Glutaryl-CoA dehydrogenase (GCDH) is an acyl-CoA dehydro­genase (ACDH) which catalyzes an intermediate step in the metabolic breakdown of lysine and tryptophan. Unlike other flavoproteins within this family, GCDH (EC 1.3.99.7) performs α,β-dehydrogenation as well as decarboxylation of its sub­strate glutaryl-CoA to yield the product crotonyl-CoA. Transfer of electrons from the glutaryl-CoA precursor to the electron-transfer flavoprotein is mediated by the cofactor flavin adenine dinucleotide (FAD) in both prokaryotic and eukaryotic electron-transport chains. Like other ACDHs, GCDH from B. pseudomallei (BpGCDH) exists as a homotetramer with tetrahedral symmetry and possesses an overall fold similar to that of the human enzyme.

Additional structures of BpGCDH resulting from this effort were obtained by soaking apo BpGCDH crystals in drops containing our Fragments of Life (FOL) ligand collection prior to data collection. All fragments identified by screening which bind BpGCDH occupy the pockets that bind the glutaryl and flavin moieties of the substrate and cofactor, respectively. In three of the four ligand-bound complexes fragment molecules occupy the binding site for the terminal glutamate of the glutaryl-coenzyme A substrate. The crystallographic water coordinated to the Arg97 side chain in the apo structure of BpGCDH remains in place when FOL544 is bound, but is displaced by FOL239 and FOL6421. In all three of these cases the Tyr373 side chain is rotated approximately 90° from its position in both the apo BpGCDH structure and the human ternary complex. This new position appears to facilitate ligand binding by providing a parallel aromatic surface that aligns with the heteroaromatic rings of all three fragments. However, a conserved backbone deviation is observed between the structure of apo BpGCDH and those of all four fragment-bound complexes in this same region. In all four fragment-bound structures Thr376 and His377 are flipped out of the α-helix observed in the apo state, partially occupying the binding pocket for the adenosine moiety of FAD. This perturbation results in a new orientation of the catalytic YEG motif. Thus, the binding of small metabolite-like ligands induces a conformation in apo crystals of BpGCDH that partially fills the FAD-binding site with protein residues.

>MAAATFHWDDPLLLDQQLADDERMVRDAAHAYAQGKLAPRVTEAFRHETTDAAIFREMGEIGLLGPTIPEQYGGPGLDYVSYGLIAREVERVDSGYRSMMSVQSSLVMVPIFEFGSDAQKEKYLPKLATGEWIGCFGLTEPNHGSDPGSMVTRARKVPGGYSLSGSKMWITNSPIADVFVVWAKLDEDGRDEIRGFILEKGCKGLSAPAIHGKVGLRASITGEIVLDEAFVPEENILPHVKGLRGPFTCLNSARYGIAWGALGAAESCWHIARQYVLDRKQFGRPLAANQLIQKKLADMQTEITLGLQGVLRLGRMKDEGTAAVEITSIMKRNSCGKALDIARLARDMLGGNGISDEFGVARHLVNLEVVNTYEGTHDIHALILGRAQTGIQAFF[4x]>MAAACRSVKGLVAVITGGASGLGLATAERLVGQGASAVLLDLPNSGGEAQAKKLGNNCVFAPADVTSEKDVQTALALAKGKFGRVDVAVNCAGIAVASKTYNLKKGQTHTLEDFQRVLDVNLMGTFNVIRLVAGEMGQNEPDQGGQRGVIINTASVAAFEGQVGQAAYSASKGGIVGMTLPIARDLAPIGIRVMTIAPGLFGTPLLTSLPEKVCNFLASQVPFPSRLGDPAEYAHLVQAIIENPFLNGEVIRLDGAIRMQP[4x];> SNAPRKDPLRHLRTREKRGPSGCSGGPNTVYLQVVAAGSRDSGAALYVFSEFNRYLFNCGEGVQRLMQEHKLKVARLDNIFLTRMHWSNVGGLSGMILTLKETGLPKCVLSGPPQLEKYLEAIKIFSGPLKGIELAVRPHSAPEYEDETMTVYQIPIHSEQRRGKHQPWQSPERPLSRLSPERSSDSESNENEPHLPHGVSQRRGVRDSSLVVAFICKLHLKRGNFLVLKAKEMGLPVGTAAIAPIIAAVKDGKSITHEGREILAEELCTPPDPGAAFVVVECPDESFIQPICENATFQRYQGKADAPVALVVHMAPASVLVDSRYQQWMERFGPDTQHLVLNENCASVHNLRSHKIQTQLNLIHPDIFPLLTSFRCKKEGPTLSVPMVQGECLLKYQLRPRREWQRDAIITCNPEEFIVEALQLPNFQQSVQEYRRSAQDGPAPAEKRSQYPEIIFLGTGSAIPMKIRNVSATLVNISPDTSLLLDCGEGTFGQLCRHYGDQVDRVLGTLAAVFVSHLHANHHTGLPSILLQRERALASLGKPLHPLLVVAPNQLKAWLQQYHNQCQEVLHHISMIPAKCLQEGAEISSPAVERLISSLLRTCDLEEFQTCLVRHCKHAFGCALVHTSGWKVVYSGDTMPCEALVRMGKDATLLIHEATLEDGLEEEAVEKTHSTTSQAISVGMRMNAEFIMLNHFSQRYAKVPLFSPNFSEKVGVAFDHMKVCFGDFPTMPKLIPPLKALFAGDIEEMEERREKRELRQVRAALLSRELAGGLEDGEPQQKRAHTEEPQAKKVRAQ;> SNAAATREFIEMWRLLGREVPEHITEEELKTLMECVSNTAKKKYLKYLYTKEKVKKARQIKKEMKAAAREEAKNIKLLETTEEDKQKNFLFLRLWDRNMDIAMGWKGAQAMQFGQPLVFDMAYENYMKRKELQNTVSQLLESEGWNRRNVDPFHIYFCNLKIDGALHRELVKRYQEKWDKLLLTSTEKSHVDLFPKDSIIYLTADSPNVMTTFRHDKVYVIGSFVDKSMQPGTSLAKAKRLNLATECLPLDKYLQWEIGNKNLTLDQMIRILLCLKNNGNWQEALQFVPKRKHTGFLEISQHSQEFINRLKKAKT

In humans, ELAC2 carries out 3′ end processing of both nucleus-encoded (nu-tRNAs) and mitochondria-encoded (mt-tRNAs) tRNAs. ELAC2 is self-sufficient for processing of nu-tRNAs but requires TRMT10C and SDR5C1 to process most mt-tRNAs. The SDR5C1 tetramer forms a base to which TRMT10C is anchored through its ‘adapter helix’ and, together, they form a platform that binds the pre-tRNA substrate through interactions with all four tRNA subdomains. ELAC2 folds into two β-lactamase domains (N-terminal domain (NTD) and endonuclease domain), which form extensive interactions with the pre-tRNA through the acceptor stem, T-arm and 3′ trailer.

To determine the molecular basis of tRNA recognition and 3′ processing by ELAC2, we reconstituted RNase Z with either the canonical pre-mt-tRNAGln (mt-RNase ZGln) or the highly degenerated pre-mt-tRNATyr substrate (mt-RNase ZTyr) and a catalytically inactive variant of ELAC2 harboring an Asp550Asn substitution (ELAC2mut)59. We, therefore, recapitulated the physiological order of events by first processing a pre-mt-tRNAGln substrate containing a 5′ leader by mt-RNase P, followed by the subsequent addition of ELAC2mut. Although TRMT10C–SDR5C1 is required only for 5′ processing but not 3′ processing of mt-tRNAGln, the pre-mt-tRNAGln remained stably bound to TRMT10C–SDR5C1 following PRORP release and association of ELAC2mut, suggesting that the TRMT10C–SDR5C1 complex also forms part of the mt-RNase Z complex for canonical mt-tRNAs. The structure of mt-RNase ZGln reveals how ELAC2 recognizes and interacts with canonical pre-tRNA substrates. The T-loop of mt-tRNAGln adopts a characteristic pentanucleotide U-turn structure, which establishes mutually stabilizing tertiary interactions with nucleobases G18 and G19 from the D-loop to form the canonical tRNA elbow. ELAC2 clamps the acceptor arm–T-arm ‘minihelix’ of pre-tRNAGln between its NTD and endonuclease domain. At the distal end of the tRNA elbow, a hydrophobic patch (residues 268–280 in helix α4) in the globular subdomain of the ELAC2 flexible arm interacts with the conserved G19–C56 tertiary base pair, stacking against its extended aromatic ring system. The first is formed near the tRNA elbow and involves hydrophobic interactions between the ELAC2 flexible arm and the TRMT10C NTD. This interface is 1.9-fold smaller than the adjacent interface between the flexible arm and the tRNA (158 Å2 between flexible arm and TRMT10C NTD versus 308 Å2 between flexible arm and tRNA), suggesting that the latter interface has the primary role in ELAC2 binding to mt-tRNAGln. Consistent with this, deletion of the ELAC2 flexible arm (Δ250–298) but not TRMT10C NTD (Δ1–124) abolished the 3′ processing of mt-tRNAGln. Taken together, these data show that ELAC2 interacts with canonical tRNAs primarily through direct protein–RNA interactions with the acceptor stem, T-arm and elbow region, while protein–protein interactions with TRMT10C are not strictly required.1-tert-butyl-3-[(3-chlorophenyl)sulfanyl]-1H-pyrazolo[3,4-d]pyrimidin-4-amine 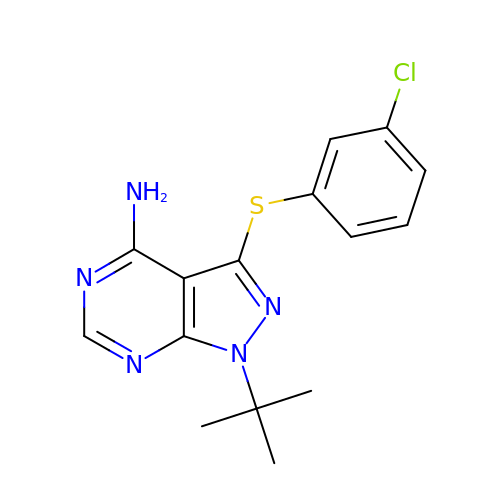| C15 H16 Cl N5 S | PNPUVQZAAVTLKS-UHFFFAOYSA-N> PIFLNVLEAIEPGVVCAGHDNNQPDSFAALLSSLNELGERQLVHVVKWAKALPGFRNLHVDDQMAVIQYSWMGLMVFAMGWRSFTNVNSRMLYFAPDLVFNEYRMHKSRMYSQCVRMRHLSQEFGWLQITPQEFLCMKALLLFSIIPVDGLKNQKFFDELRMNYIKELDRIIACKRKNPTSCSRRFYQLTKLLDSVQPIARELHQFTFDLLIKSHMVSVDFPEMM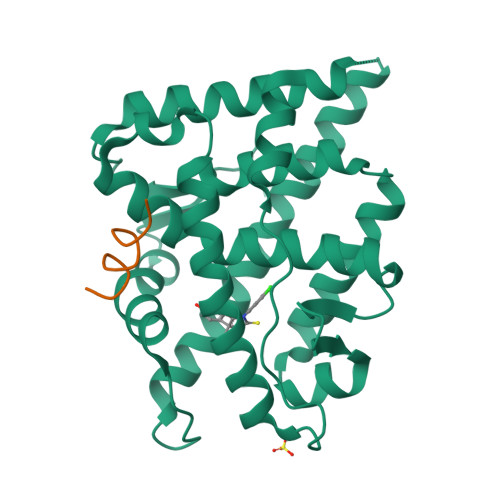AEIISVQVPKILSGKVKPIYFHTQ;> GAFQNLFQSVR> MGSSHHHHHHSSGRENLYFQGHMQLSHRPAE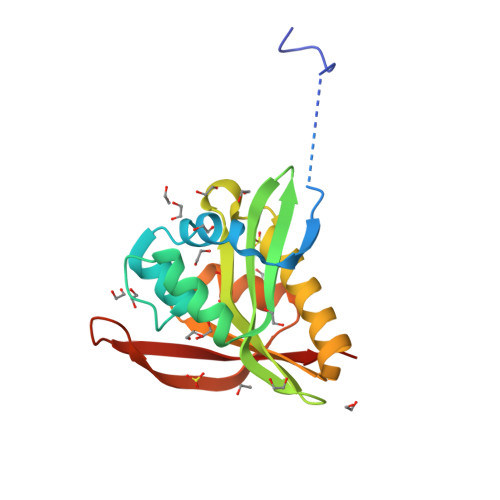TGDLETVAGFPQDRDELFYCYPKAIWPFSVAQLAAAIAERRGSTVAVHDGQVLGFANFYQWQHGDFCALGNMMVAPAARGLGVARYLIGVMENLAREQYKARLMKISCFNANAAGLLLYTQLGYQPRAIAERHDPDGRRVALIQMDKPLEP>[8x]MGSSHHHHHHMSNVTVSAFTVDKSISEEHVLPSSFIPGSGNIFPKFTSAIPKTAWELWYFDGISKDDKSSIVIGVTRNAEGLKHGGFKVQVFVIWADERTWHRDLFFPESVVSINESGVTDGIWKDAT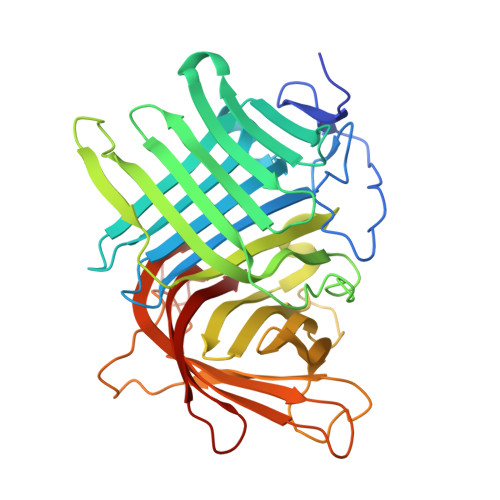SNSSISFSCAGDLSKASLVFDVPGVVQGDMHLEALPGDTGLDTDARLGPSVYYVRPIGRASVKAQLSLYSSDATAAEQFSLGTSANGGMDRVWSPLSWPQVMTESYYLRTQVGPYAMQIMRIFPPAGSEDQPSTMARLYREGQLVCVAQHVVTREDALMTHDSLILSKQDNSDSEDVVTGGYRDKNTGYTVEFVEKGNEGQRWKFQVRHERIIWNTPTSRPGPDATGNTGFVEVLCGGTIGESYEGVGTGGQCELS>MGDSEEPVVTPHAPEFAFDPTDPWTETFQRGLEIAGLGGKRVYEVGIGTGINVAFMLQICEAALVSGSDLDPRLAGLAERNVRDLAPRRADRFHPVEGAVSLIDTPEARAQVGRSDVIVGCLPQVGEPDDVRLRAFRTAQAAALAAGADTRDEDHIAHYYPWAEFDSYPFNSVGLGLNEALLRRTRATAPAADVVLNFGARVG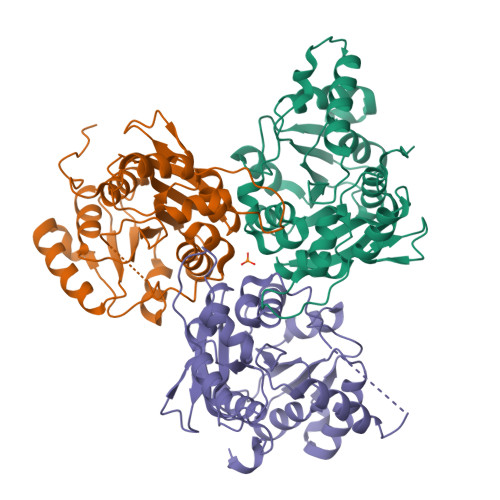SAVLFELFEANGYVPEKLHSQIVLQHAGTDISFFVALENALAQTGLEREFTCEFYGDPEGATRLSATEAQALVDTDSAAEIYHEVCVIRGRPALSENDPSDS[3x]>QKEQHSQLNQTKIAYEQRLLNDLEDMDDPLDLFLDYMIWISTSYIEVDSESGQEVLRSTMERCLIYIQDMETYRNDPRFLKIWIWYINLFLSNNFHESENTFKYMFNKGIGTKLSLFYEEFSKLLENAQFFLEAKVLLELGAENNCRPYNRLLRSLSNYEDRLREMNIVENQNSVPDSRERLKGRLIYRTAPFFIRKFLTSS[2x]

The interaction of the central mitotic checkpoint component BUB1 with the mitotic kinetochore protein Blinkin is required for the kinetochore localization and function of BUB1 in the mitotic spindle assembly checkpoint, the regulatory mechanism of the cell cycle that ensures the even distribution of chromosomes during the transition from metaphase to anaphase. Sequence comparison of BUB1 and BUBR1 shows that these proteins share a common architecture: a conserved N-terminal region, a central nonconserved region that contains the binding region for other mitotic checkpoint components such as BUB3, and a C-terminal serine/threonine kinase domain. The N-terminal region mediates the binding of Hs-BUB1 to the mitotic kinetochore protein Blinkin (a protein also commonly referred to as AF15q14); the interaction is essential for the kinetochore localization of this protein and its function in cell cycle arrest induced by SAC activation (Kiyomitsu et al., 2007). The structure shows that a divergent triple tandem arrangement of the TPR motif constitutes a suitable structural framework for the physical linkage of BUB1 to interacting partners.

The crystal structure of the N-terminal region of Sc-BUB1(29-230) from budding yeast was solved at 1.74 Å resolution, and contains two molecules of BUB1 in the asymmetric unit, related by a noncrystallographic two-fold axis, forming a homodimer. The two protomers are associated primarily by hydrogen bonds and van der Waals interactions and involve clusters of conserved residues E52-P57, M98-K109, and R175-R182. Salt bridges between the oxygen atom of residue D53 of one protomer and the nitrogen atoms (NH1, NH2) of R179 and R182 of the other, as well as between D55 of one protomer and K109, R175, and R179 of the other, contribute further to the stability of the homodimer. The structure of the Sc-BUB1(29-230) protomer consists of ten α helices (H1–H10) that contribute three major features: a single α helix (H1), a tandem repeat of three units of the tetratricopeptide (TPR) motif (H2-H7), and a C-terminal region encompassing three α helices (H8-H10). Each TPR unit (TPR1, TPR2, and TPR3, numbered from the N terminal) comprises two antiparallel α helices, arranged as a helix-turn-helix hairpin. The uniform arrangement of neighboring α helices gives rise to the formation of a right-handed superhelical structure with a continuous concave surface on one side and a contrasting convex surface on the other. The amphipathic helix 8, which encompasses residues Y177 to M194, has the features of a “capping helix. Helices H9 and H10 lie parallel to the long axis of the TPR core, establishing extensive polar contacts with TPR helices H3, H4, H5, H6, and H7. The analysis of the crystal structure of Sc-BUB1(29-230) strongly suggests that the impaired interaction between these Hs-BUB1 mutants and Blinkin is due to the disruption of stabilizing interactions among α helices of the TPR units.>GSHMTSSANEDMPVERILEAELAVEPKTETYVEANMGLNPSSPNDPVTNICQAADKQLFTLVEWAKRIPHFSELPLDDQVILLRAGWNELLIASFSHRSIAVKDGILLATGLHVHRNSAHSAGVGAIFDRVLTELVSKMRDMQMDKTELGCLRAIVLFNPDSKGLSNPAEVEALREKVYASLEAYCKHKYPEQPGRFAKLLLRLPALRSIGLKCLEHLFFFKLIGDTPIDTFLMEMLE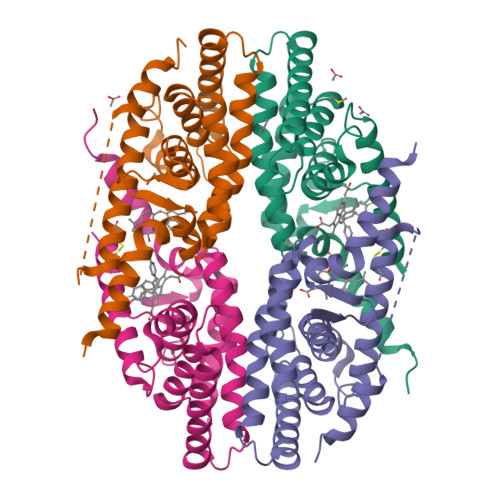APHQMT[4x]>SRCTHLENRDFVTGTQGTTRVTLVLELGGCVTITAEGKPSMDVWLDAIYQENPAKTREYCLHAKLSDTKVAARCPTMGPATLAEEHQGGTVCKRDQSDRGWGNHCGLFGKGSIVACVKAACEAKKKATGHVYDANKIVYTVKVEPHTGDYVAANETHSGRKTASFTISSEKTILTMGEYGDVSLLCRVASGVDLAQTVILELDKTVEHLPTAWQVHRDWFNDLALPWKHEGAQNWNNAERLVEFGAPHAVKMDVYNLGDQTGVLLKALAGVPVAHIEGTKYHLKSGHVTCEVGLEKLKMKGLTYTMCDKTKFTWKRAPTDSGHDTVVMEVTFSGTKPCRIPVRAVAHGSPDVNVAMLITPNPTIENNGGGFIEMQLPPGDNIIYVGELSHQWFQKGSSIGRVFQKTKKGIERLTVIGEHAWDFGSAGGFLSSIGKAVHTVLGGAFNSIFGGVGFLPKLLLGVALAWLGLNMRNPTMSMSFLLAGGLVLAMTLGVGA[3x];>[3x]TVRKERDGSTVIRAEGKDAATQVRVENGTCVILATDMGSWCDDSLSYECVTIDQGEEPVDVDCFCRNVDGVYLEYGRCGKQEGSRTRRSVLIPSHAQGELTGRGHKWLEGDSLRTHLTRVEGWVWKNKLLALAMVTVVWLTLESVVTRVAVLVVLLCLAPVYA

The envelope of immature TBEV particle contains 180 copies of each M protein precursor (prM) and E forming heterodimers. The prM protein stabilizes E, preventing premature virus activation and its fusion at low pH with the membranes of the trans-Golgi network (TGN). Flavivirus maturation occurs at mildly acidic pH, when host protease furin cleaves the prM protein to a pr peptide that will later dissociate from the particle and the M protein that remains in the particle, resulting in infectious viruses. Our atomic models of the major viral components, the E and prM proteins, indicate that the pr domains of prM have a critical role in holding the heterohexameric prM3E3 spikes in a metastable conformation.

To acquire a comprehensive understanding of the immature TBEV particle structure, we investigated three strains: Hypr, Neudoerfl, and Kuutsalo-14. We observed a 1.0-Å root-mean-square deviation (RMSD) between Kuutsalo-14 and Neudoerfl atomic models for the Cα of prM and E ectodomains. The regions contributing to higher RMSD are in β sheets of E-DIII and loops. The RMSD of the Cα of the membrane-associated helices was 2.1 Å, reflecting the lower resolution of these regions. Thus, the prM3E3 arrangement of the immature TBEV particle is mostly maintained by the interactions between pr domains within the prM3E3 spike. We were able to build the linker along the E protein up to Gly98, including the conserved 85-Arg Thr Arg Arg-88 furin recognition site. The cleavage of prM at Arg88 splits it into pr peptide (residues 1 to 88) and M protein (residues 89 to 162) and is a crucial step of TBEV maturation. Within the immature particle context, the furin cleavage sites are located “inside” the spike and are inaccessible to the globular 88-kDa furin without a conformational rearrangement of the spike. A strictly conserved His95 from the prM linker interacts with the E hydrophobic pocket. This His is located within 4.5 Å of the conserved His216 in E, and we speculate that when protonated, these residues cooperate to trigger exposure of the loop containing the furin cleavage site to allow the conformational changes leading to proteolysis.> MKTFIFLALLGAAVAFPVDDDDKIVGGYTCGANTVPYQVSLNSGYHFCGGSLINSQWVVSAAHCYKSGIQVRLGEDNINVVEGNEQFISASKSIVHPSYNSNTLNNDIMLIKLKSAASLNSRVASISLPTSCASAGTQCLISGWGNTKSSGTSYPDVLKCLKAPILSDSSCKSAYPGQITSNMFCAGYLEGGKDSCQGDSGGPVVCSGKLQGIVSWGSGCAQKNKPGVYTKVCNYVSWIKQTIASN

The RoboDiff forms the core of the services offered on the ESRF beamline MASSIF-1 and, thus far, has been used to mount, characterize and collect diffraction data from over 20 000 samples since September 2014. In all three cases diffraction images were indexed and integrated using XDS and reduced using AIMLESS.

For trypsin, the structure was solved by molecular replacement (MR) using MOLREP.>MFNRPILFDIVSRGSTADLDGLLPFLLTHKKRLTDEEFREPSTGKTCLPKALLNLSNGRNDTIPVLLDIAERTGNMREFINSPFRDIYYRGQTALHIAIERRCKHYVELLV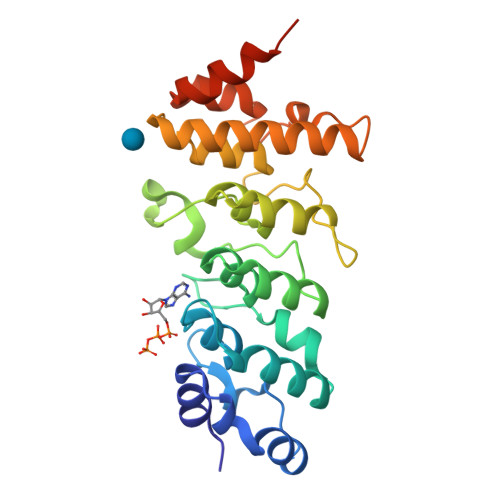AQGADVHAQARGRFFQPKDEGGYFYFGELPLSLAACTNQPHIVNYLTENPHKKADMRRQDSRGNTVLHALVAIADNTRENTKFVTKMYDLLLLKCARLFPDSNLEAVLNNDGLSPLMMAAKTGKIGIFQHIIRREVTDEAAAHHHHHH[2x]> MKPTMAILERISKNSQENIDEVFTRLYRYLLRPDIYYVAYQNLYSNKGASTKGILDDTADGFSEEKIKKIIQSLKDGTYYPQPVRRMYIAKKNSKKMRPLGIPTFTDKLIQEAVRIILESIYEPVFEDVSHGFRPQRSCHTALKTIKREFGGARWFVEGDIKGCFDNIDHVTLIGLINLKIKDMKMSQLIYKFLKAGYLENWQYHKTYSGTPQGGILSPLLANIYLHELDKFVLQLKMKFDRESPERITPEYRELHNEIKRISHRLKKLEGEEKAKVLLEYQEKRKRLPTLPCTSQTNKVLKYVRYADDFIISVKGSKEDCQWIKEQLKLFIHNKLKMELSEEKTLITHSSQPARFLGYDIRVRRSGTIKRSGKVKKRTLNGSVELLIPLQDKIRQFIFDKKIAIQKKDSSWFPVHRKYLIRSTDLEIITIYNSELRGICNYYGLASNFNQLNYFAYLMEYSCLKTIASKHKGTLSKTISMFKDGSGSWGIPYEIKQGKQRRYFANFSECKSPYQFTDEISQAPVLYGYARNTLENRLKAKCCELCGTSDENTSYEIHHVNKVKNLKGKEKWEMAMIAKQRKTLVVCFHCHRHVIHKHK

In this work, we develop functionalized graphene grids with various charges via a dediazoniation reaction for cryo-EM specimen preparation. By applying onto three different types of macromolecules, we demonstrate that the high-yield charged graphene grids bring macromolecules away from the AWI and enable adjustable particle-orientation distribution for more robust single particle cryo-EM structural determination. In this work, to overcome the graphene functionalization and transfer challenges and solve the preferential orientation problem, we develop a method to produce robust graphene grids functionalized with different electrostatic charges, which provide various electrostatic interaction interface for target macromolecules to bind in and enrich orientations. The charged graphene grids provide different surfaces for protein molecules or macromolecule complexes to interact with, based on the target molecule’s surface charge properties, therefore allowing multiple orientations on various charged graphene grids and avoiding impairment by the AWI.

We lastly applied the charged graphene grids to the group IIA intron RNP complex, L1.LtrB in Lactococcus lactis, which is composed of an RNA chain and a polypeptide chain. The cryo-EM structure determination of L1.LtrB RNP was largely impaired by the notorious preferred orientation problem on either holey carbon films or conventional supporting films. We used the NFG and SFG to prepare the cryo-EM specimen of Ll.LtrB RNP and found various views on the NFG and SFG, in contrast to only one dominant view on conventional graphene treated by residual air-glow discharge. The analysis of the orientational distribution showed that the negatively charged RNA chain plays a key role when interacting with the NFG while the polypeptide chain with relatively positive charges directs the interaction with the SFG. The other notable thing is that we picked 972,269 particles from air-glow-treated conventional graphene support but only 55,783 particles were kept for the final 3D reconstruction. This means that the useful particle proportion on the conventional graphene support is 5.7%, much lower than that on SFG (35.7%) or NFG (23.5%), indicating a more friendly interacting interface with Ll.LtrB RNP particles on our modified graphene. By using a combination of particle images from the two differently charged graphene grids, we were able to obtain the reconstruction of Ll.LtrB RNP complex at 3.2-Å resolution. This marked the highest resolution of the endogenously purified group II intron RNP, where the bases and metal ions in the catalytic center can be clearly recognized.>GPGSMTKTWTLKKHFVGYPTNSDFELKTSELPPLKNGEVLLEALFLTVDPYMRVAAKRLKEGDTMMGQQVAKVVESKNVALPKGTIVLASPGWTTHSISDGKDLEKLLTEWPDTIPLSLALGTVGMPGLTAYFGLLEICGVKGGETVMVNAAAGAVGSVVGQIAKLKGCKVVGAVGSDEKVAYLQKLGFDVVFNYKTVESLEETLKK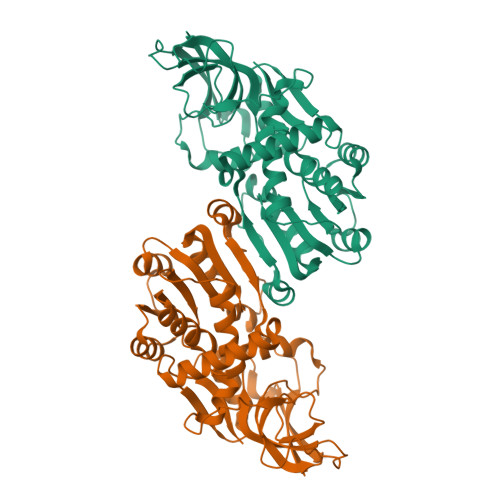ASPDGYDCYFDNVGGEFSNTVIGQMKKFGRIAICGAISTYNRTGPLPPGPPPEIVIYQELRMEAFVVYRWQGDARQKALKDLLKWVLEGKIQYKEYIIEGFENMPAAFMGMLKGDNLGKTIVKA[2x]(2S,3S)-3-(4-fluorophenyl)-2,3-dihydroxypropanoic acid | C9 H9 F O4 | 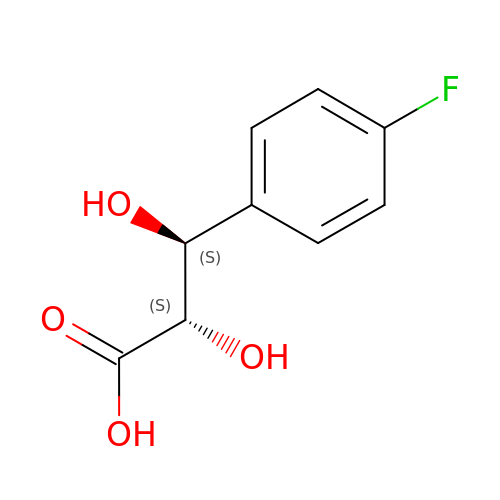DWYLYIVEFVSGCP-YUMQZZPRSA-N>[2x]AHSIRVDGDIILGGLFPVHAKGERGVPCGELKKEKGIHRLEAMLYAIDQINKDPDLLSNITLGVRILDTCSRDTYALEQSLTFVQALIEKDASDVKCANGDPPIFTKPDKISGVIGA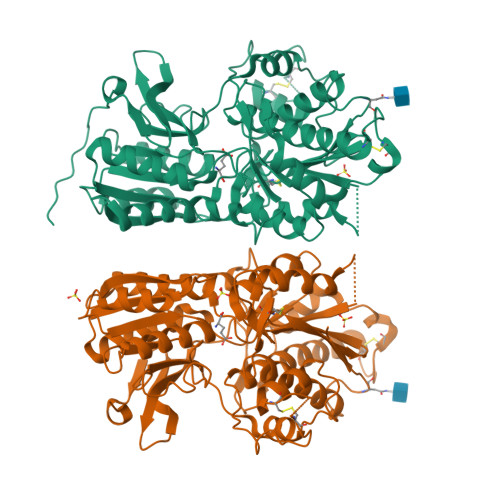AASSVSIMVANILRLFKIPQISYASTAPELSDNTRYDFFSRVVPPDSYQAQAMVDIVTALGWNYVSTLASEGNYGESGVEAFTQISREIGGVSIAQSQKIPREPRPGEFEKIIKRLLETPNARAVIMFANEDDIRRILEAAKKLQQSGHFLWIGSDSWGSKIAPVYQQEEIAEGAVTILPKRASIDGFDRYFRSRTLANNRRNVWFAEFWEENFGCKLGSHGKRNSHIKKCTGLERIARDSSYEQEGKVQFVIDAVYSMAYALHNMHKDLCPGYIGLCPRMSTIDGKELLGYIRAVNFNGSAGTPVTFNENGDAPGRYDIFQYQITNKSTEYKVIGHWTNQLHLKVEDMQWAHREHTHPASE8-[[(1~{S},2~{R},3~{R},5~{R})-2-[2-[1,1-bis(oxidanylidene)thian-4-yl]ethyl]-8-azabicyclo[3.2.1]octan-3-yl]amino]-3-methyl-5-(5-methylpyridin-3-yl)-1~{H}-quinolin-2-one | C30 H38 N4 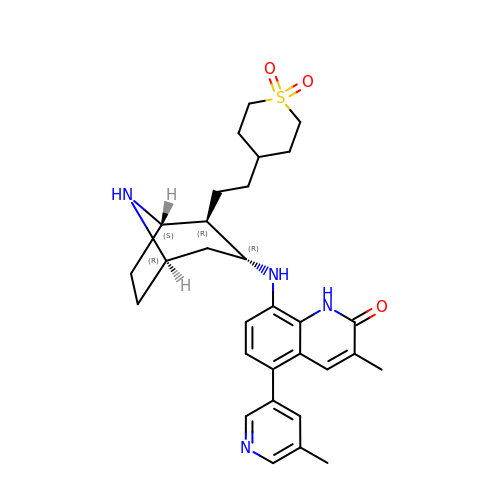O3 S | RYLMNRNKGQACDG-PVRUFOIFSA-N Milano is a contractile tail bacteriophage that infects the pathogenic plant bacterium Agrobacterium tumefaciens, an important tool that is widely used in genetic manipulations of plants. The contractile tail of Agrobacterium tumefaciens bacteriophage Milano is flexible and bent to varying degrees, which sets it apart from other contractile tail-like systems. A contractile sheath and rigid tube assembly is a widespread apparatus used by bacteriophages, tailocins, and the bacterial type VI secretion system to penetrate cell membranes. In this mechanism, contraction of an external sheath powers the motion of an inner tube through the membrane.

To explore the fate of sheath disulfide bonds upon contraction, we solved the atomic structure of the contracted sheath. The structures of the sheath subunit in the contracted and extended states are similar and can be superimposed with an RMSD of 0.7 Å between 347 pruned Cα atoms out of a total of 491 Cα atoms with an RMSD of 3.9 Å. The larger all-atom RMSD arises from the different relative orientations of the linker arms invading the neighboring subunits’ SHD. The rearrangement of sheath subunits upon contraction resembles that found in other CISs (roughly, each subunit rotates and moves radially), and the integrity of the two-dimensional mesh created by the sheath linker arms is preserved. Upon full contraction, the Milano sheath subunit rotates by ~12° and moves by ~13 Å radially. Two of the three disulfide bonds that crosslink sheath subunits to each other are retained in the contracted sheath (Cys14SHD–Cys244SBD and Cys216SBD–Cys327SBD) whereas the Cys47SBD–Cys182SED bond is broken. This suggests that the disulfide bond Cys47SBD–Cys182SED needs to be released to allow for the rotation and radial movement of sheath subunits during contraction. We could induce contraction by a mixture of guanidine hydrochloride (3M) and dithiothreitol (DTT, 5 mM), a reducing agent. In the contracted (post-attachment) state, the tails were straight.

> MAQDALSDGFVRLCIDPSLNFFGEGCKILVEGQMTDDGSATPDAVTCVTSELDIIERFGQGSVLTESLRKVFCTCKSGVSVYALPREDAAAGVKAVYTLTIAGPATTDGRVQLYMGEAEYAVDIGVDAGDTATDIAAAIVAAISPDFPYAATAAAGVITLTARNAGTIGNHLSVIYTNLGSCTSVTPEGVTVTFAQTTAGSVNPTPNDYATVVNECCFAVYVLSSDDTDWQENLRDWIRSAWDCSKPQCFGHGYVFNKGTLGQVLADGDNSAELSRLALPTTYPVLPYLTNAAYGALSACSTCNNPELNIQGQTFGLLSCINMPESCTPGWTFGEVTQLQANGFVVSGPSTTSGQGNYTSPYIYNDVTNYLRDEKNRPNATFRDASSRRLAAATGVALAEFLQQFNGLAVFTKNTNIRTGIIGTNPRLMLGKIRKWAQDNVGTLFSEFDNINEDIQLLTDFEVQPKCVGQPGIFHLNMRYRPPVRGARINVNMAPALFDNCDR> MVRTITVASGKGGTGKTTITANLGVALAQLGHDVTIVDADITMANLELILGMEGLPVTLQNVLAGEARIDEAIYVGPGGVKVVPAGVSLEGLRKANPEKLEDVLTQIMESTDILLLDAPAGLERSAVIAIAAAQELLLVVNPEISSITDGLKTKIVAERLGTKVLGVVVNRITTLGIEMAKNEIEAILEAKVIGLIPEDPEVRRAAAYGKPVVLRSPNSPAARAIVELANYIAGGAKKKVPAEVKEKKKEGALAKM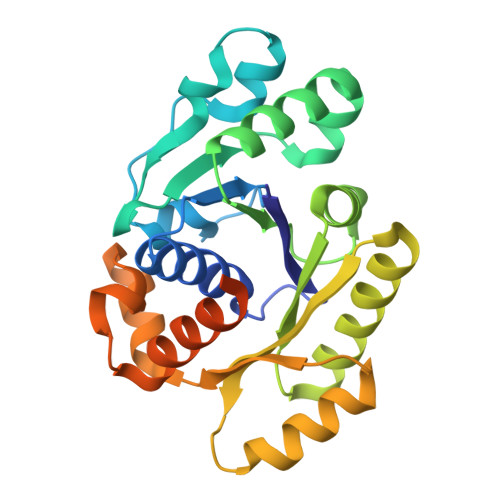LRIFRRR> HPYYLRSFLVVLKTVLENEDDMLLFDEQEKGIVTKFYQLSATGQKLYVRLFQRKLSWIKMTKLEYEEIALDLTPVIEELTNAGFLQTESELQELSEVLELLSAPELKSLAKTFHLVNPNGQKQQLVDAFLKLAKQHSVCTWGKNKPGIGAVILKRAKALAGQSVRICKGPRAVFSRILL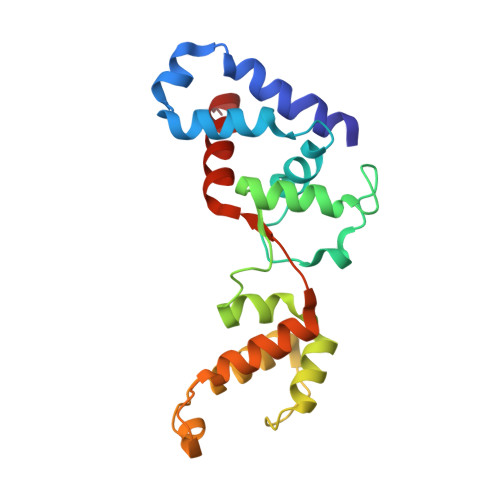LFSLT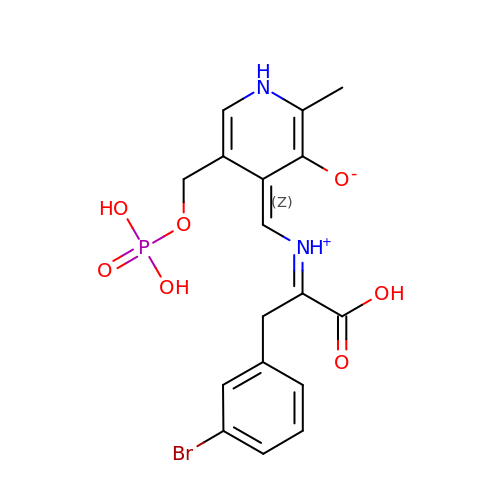(4Z)-4-({[(1E)-2-(3-bromophenyl)-1-carboxyethylidene]azaniumyl}methylidene)-2-methyl-5-[(phosphonooxy)methyl]-1,4-dihydropyridin-3-olate | C17 H18 Br N2 O7 P | QODYJTOPURJJAH-MTTBYZIPSA-N>AGFQLNEFSSSGLGRAYSGEGAIADDAGNVSRNAALITMFDRPTFSAGAVYIDPDVNISGTSPSGRSLKADNIAPTAWVPNMHFVAPINDQFGWGASITSNYGLATEFNDTYAGGSVGGTTDLETMNLNLSGAYRLNNAWSFGLGFNAVYARAKIERFAGDLGQLVAGQIMQSPAGQTQQGQALAATANGIDSNTKTAHLNGNQWGFGWNAGILYELDKNNRYALTYRSEVKIDFKGNYSSDLNRAFNNYGLPIPTATGGATQSGYLTLNLPEMWEVSGYNRVDPQWAIHYSLAYTSWSQFQ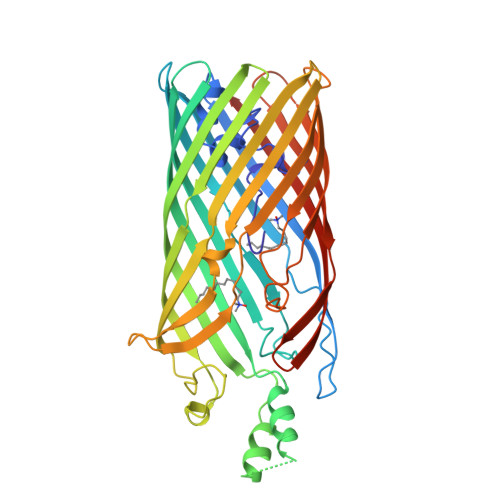QLKATSTSGDTLFQKHEGFKDAYRIALGTTYYYDDNWTFRTGIAFDDSPVPAQNRSISIPDQDRFWLSAGTTYAFNKDASVDVGVSYMHGQSVKINEGPYQFESEGKAWLFGTNFNYAFHHHHHH[3x]> MIAGTPPHSTMERGGDRDIVVTGARNQFAPDLEPGGSVSCMRSSLSFLSLIFDVGPRDVLSAEAIEGCLVEGGEWTRATAGPGPPRMCSIVELPNFLEYPGARGGLRCVFSRVYGEVGFFGEPAAGLLETQCPAHTFFAGPWALRPLSYTLLTIGPLGMGLFRDGDTAYLFDPHGLPEGTPAFIAKVRAGDMYPYLTYYTRDRPDVRWAGAMVFFVPSGPEPAAPADLTAAALHLYGASETYMQDEAFSERRVAITHPLRGEIAGLGEPCVGVGPREGGGGPGPHPPTAAQSPPPTRARRDDRASETSRGTAGPSAKPEAKRPNRAPDDVWAVALKGTPPTDPPSADPPSAIPPPPPSAPKTPAAEAAEEDDDDMRVLEMGVVPVGRHRARYSAGLPKRRRPTWTPPSSVEDLTSGEKTKRSAPPAKTKKKSTPKGKTPVGAAVPASVPEPVLASAPPDPAGPPVAEAGEDDGPMVPASSQALEALKTRRSPEPPGADLAQLFEAHPNVAATAVKFTACSATLAREVAACSRLTISALRSPYPASPGLLELCVIFFFERVLAFLIENGARTHTQAGVAGPAAALLEFTLSMLPRKTAVGDFLASTRLSLADVAAHLPLVQHVLDENSLIGRLALAKLILVARDVIRETDAFYGELADLELQLRAAPPANLYTRLGEWLLERSQAHPDTLFAPATPTHPEPLLYRVQALAKFARGEEIRVEAEDRQMREALDALARGVDAVSQHAGPLGVMPAPAGAAPQGAPRPPPLGPEAVQVRLEEVRTQARRAIEGAVKEYFYRGAVYSAKALQASDNNDRRFHVASAAVVPVVQLLESLPVFDQHTRDIAQRAAIPAPPPIATSPTAILLRDLIQRGQTLDAPEDLAAWLSVLTDAANQGLIERKPLDELARSIRDINDQQARRSSGLAELRRFDALDAALGQQLDSDAAFVPAPGASPYPDDGGLSPEATRMAEEALRQARAMDAAKLTAELAPDARARLRERARSLEAMLEGARERAKVARDAREKFLHKLQGVLRPLPDFVGLKACPAVLATLRASLPAGWSDLPEAVRGAPPEVTAALRADMWGLLGQYRDALEHPTPDTATALSGLHPSFVVVLKNLFADAPETPFLLQFFADHAPIIAHAVSNAINAGSAAVATADPASTVDAAVRAHRVLVDAVTALGAAASDPASPLAFLAAMADSAAGYVKATRLALDARGAIAQLTTLGSAAADLVVQVRRAANQPEGEHASLIQAATRATTGARESLAGHEGRFGGLLHAEGTAGDHSPSGRALQELGKVIGATRRRADELEAAIADLREKMAAQRARSSHERWAADVEAVLDRVESGAEFDVVELRRLQALAGTHGYNPRDFRKRAEQALGTNAKAVTLALETALAFNPYTPENQRHPMLPPLAAIHRIDWSAAFGAAADTYADMFRVDTEPLARLLRLAGGLLERAQANDGFIDYHEAVLHLSEDLGGVPALRQYVPFFQKGYAEYVDIRDRLDALRADARRAIGSVALDLAAAAEEISAVRNDPAAAAELVRAGVTLPCPSEDALVACVAALERVDQSPVKDTAYADYVAFVTRQDLADTKDAVVRAKQQRAEATERVTAGLREVLAARERRAQLEAEGLANLKTLLKVVAVPATVAKTLDQARSAEEIADQVEILLDQTEKARELDVQAVAWLEHAQRTFETHPLNAASGDGPGLLTRQGARLQALFDTRRRVEALRRSLEEAEAEWDEVWGRFGRVRGGAWKSPEGFRAACEQLRALQDTTNTVSGLRAQRDYERLPAKYQGVLGAKSAERAGAVEELGGRVAQHADLSARLRDEVVPRVAWEMNFDTLGGLLAEFDAVAGDLAPWAVEEFRGARELIQRRMGLYSAYAKATGQTGAGAAAAPAPLLVDLRALDARARASAPPGQEADPQMLRRRGEAYLRVSGGPGPLVLREATSTLDRPFAPSFLVPDGTPLQYALCFPAVTDKLGALLMCPEAACIRPPLPTDTLESASTVTAMYVITVINRLQLALSDAQAANFQLFGRFVRHRQARWGASMDAAAELYVALVATTLTREFGCRWAQLEWGGDAAAPGPPLGPHSSTRHRVSFNENDVLVALVASSPEHIYTFWRLDLVRQHEYMHLTLPRAFQNAADSMLFVQRLTPHPDARIRVLPVFSTGGPPTRGLMFGTRLADWRRGKLSETDPLAPWRSVPELGTERGAALGKLSPAQALAAVSVLGRMCLPSTALAALWTCMFPDDYTEYDSFDALLTARLESGQTLSPSGGREA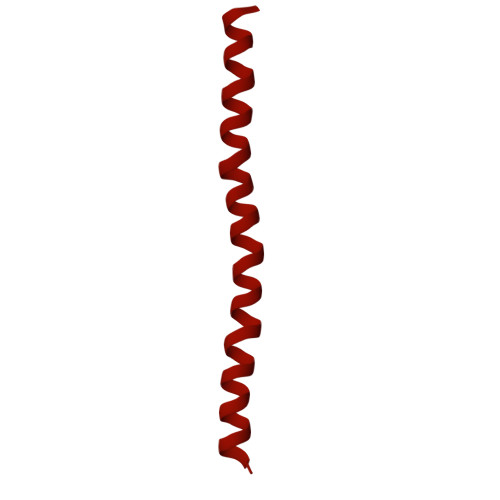SPPAPPNALYRPTGQHVAVPAAATHRTPAARVTAMDLVLAAVLLGAPVVVALRNTTAFSRESELELCLTLFDSRARGPDAALRDAVSSDIETWAVRLLHADLNPIENACLAAQLPRLSALIAERPLARGPPCLVLVDISMTPVAVLWENPDPPGPPDVRFVGSEATEELPFVAGGEDVLAASATDEDPFLARAILGRPFDASLLSGELFPGHPVYQRAPDDQSPSVPNPTPGPADLVGTEGSLGPGSLAPTLFTDATPGEPVPPRMWAWIHGLEELASDDSGGPAPLLAPDPLSPTADQSVPTSQCAPRPPGPAVTAREARPGVPAESTRPAPVGPRDDFRRLPSPQSSPAPPDATAPRPPASSRASAASSSGSRARRHRRARSLARATQASATTQGWRPPALPDTVAPVTDFARPPAPPKPPEPALHALVSGVPLPLGPQFAGQASPALPIDPVPPPVATGTVLPGGENRRPPLTSGPAPTPPRVPVGGPQRRLTRPAVASLSESRESLPSPWDPADPTAPVLGRNPAEPTSSSPAGPSPPPPAVQPVTPPPTSGPPPTYLTLEGGVTPGGPVSRRPTTRQPVATPTTSARPRGHLTVNRLSAPQPQPQPQPQPQPQPQPQPQPQPQPQPQPQNGHVAPGEYPAVRFRAPQNRPSVPASASSTNPRTGSSLSGVSSWASSLALHIDATPPPVSLLQTLYVSDDEDSDTTSLFLSDSEAEALDPLPREPHSPITNEPFSALSADDSQEVTRLQFGPPPVSANAVLSRRYVQRTGRSALAVLIRACYRLQQQLQRTRRALLHHSDAVLTSLHHVRMLLG> APIPGVMPIGNYVSLYVML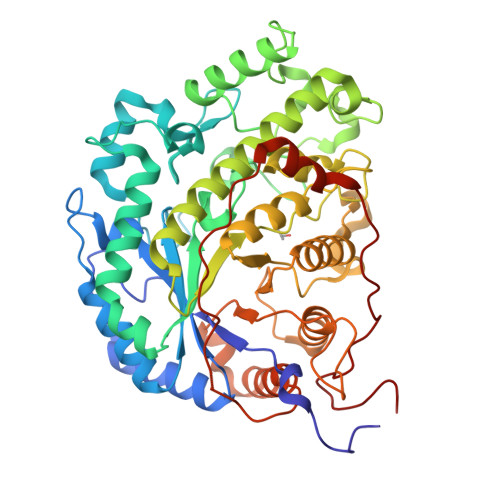PLGVVNADNVFPDKEKVEDELKQVKAGGCDGVMVDVWWGIIEAKGPKQYDWSAYRELFQLVKKCGLKIQAIMSFHQCGGNVGDAVFIPIPQWILQIGDKNPDIFYTNRAGNRNQEYLSLGVDNQRLFQGRTALEMYRDFMESFRDNMADFLKAGDIVDIEVGCGAAGELRYPSYPETQGWVFPGIGEFQCYDKYMVADWKEAVKQAGNADWEMPGKGAGTYNDTPDKTEFFRPNGTYKTDMGKFFLTWYSNKLIIHGDQVLEEANKVFVGLRVNIAAKVSGIHWWYNHVSHAAELTAGFYNVAGRDGYRPIARMLARHHATLNFTCLEMRDSEQPAEAKSAPQELVQQVLSSGWKEYIDVAGENALPRYDATAYNQMLLLVRPNGVNLNGPPKLKMSGLTYLRLSDDLLQTDNFELFKKFVKKMHADLDPSPNAISPAVLERSNSAITIDELMEATKGSRPFPWYDVTDMPVDGSNPFD> KPL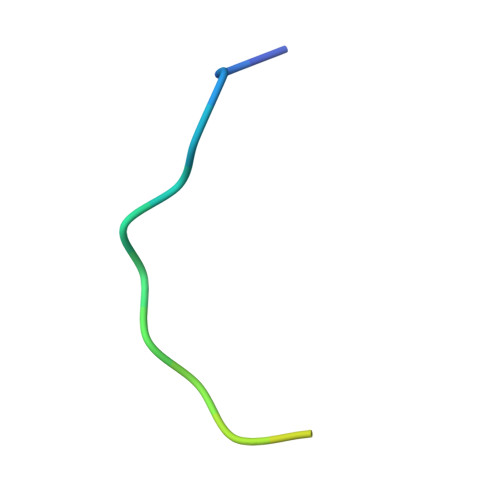QVAAVDSSVPRTAELAG>SGAFEDRDPTQFEERHLKFLQQLGKGNFGSVEMCRYDPLQDNTGEVVAVKKLQHSTEEHLRDFEREIEILKSLQHDNIVKYKGVCYSAGRRNLKLIMEYLPYGSLRDYLQKHKERIDHIKLLQYTSQICKGMEYLGTKRYIHRDLATRNILVENENRVKIGDFGLTKVLPQDKEYYKVKEPGESPIFWYAPESLTESKFSVASDVWSFGVVLYELFTYIEKSKSPPAEFMRMIGNDKQGQMIVFHLIELLKNNGRLPRPDGCPDEIYMIMTECWNNNVNQRPSFRD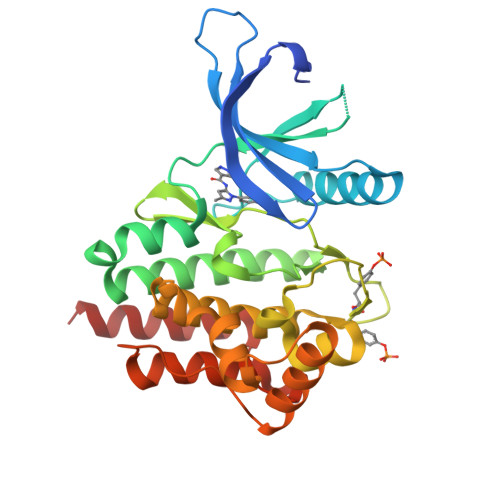LALRVDQIRDNMAG[2x]>[4x]MDVKVQYLCENTQTSTQEIKGKFNIVNTGNRDYSLKDIVLRYYFTKEHNSQLQFICSYTPIGSG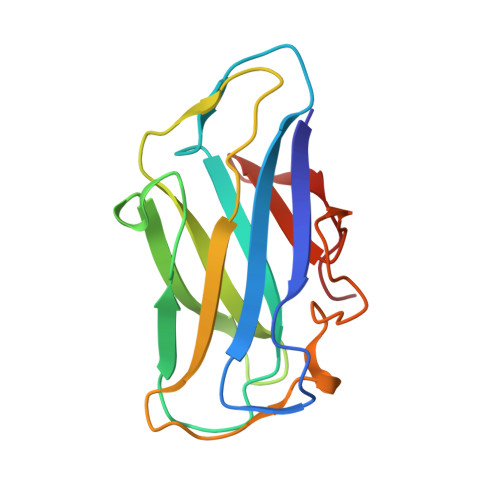NLIPSFGGSGDEHYLQLEFKDVKLPAGGQTGEIQFVIRYADNSFHDQSNDYSFDPTIKAFQDYGKVTLYKNGELVWGTPPG> SPHNPIS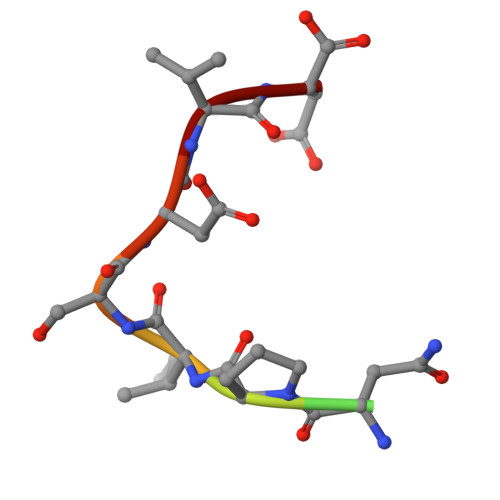DVD> EAMAKVEEVQKVVKELEKELGELDKVPSYGDAQDYSYQKALWEEFLRIGKDNMDYASKMKADDKFFHKVKGDLNDFKYQIKVENYIRQVAELRKKYPGDNTIEEEYNAHLKQD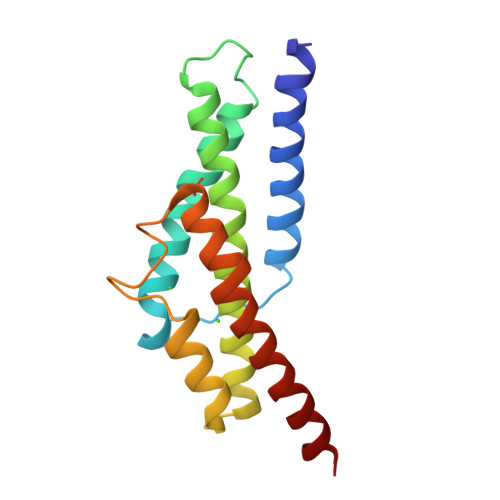EGKSIASQEGATLRDYVDREASEAMGRIKQRVAELEILEHH>HSSGLVPRGSHMSQERILDGEEDEINHKIFDLKRTLKDNLPLDRDFIDRLKRYFKDPSDQVLALRELLNEKDLTAEQVELLTKIINEIISGSEKSVNAGINSAIQAKLFGNKMKLEPQLLRACYRGFIMGNISTTDQYIEWLGNFGFNH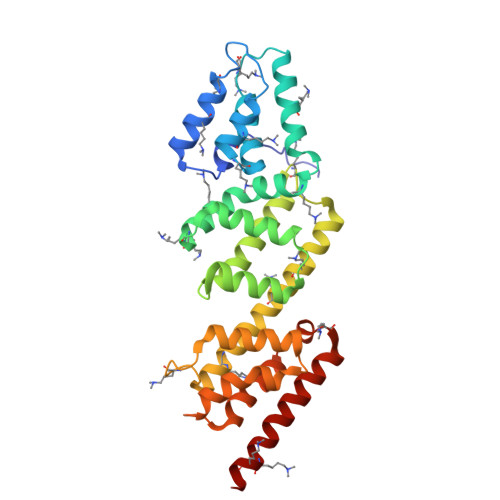RHTIVNFVEQSLIVDMDSEKPSCNAYEFGFVLSKLIAIKMIRTSDVIFMKKLESSSLLKDGSLSAEQLLLTLLYIFQYPSESEQILTSVIEVSRASHEDSVVYQTYLSSVNESPHDIFKSESEREIAINILRELVTSAYKKELSR[2x]> KNSINTIKLIDDIIALHNDPKGNKLLWNDNWQDKIINRDLANIFEKIDESVSELGGLEMYQEMVGVNPYDPTEPVCGLSAQNIFKLMTEGEHAVDPVEMAQTGKIDGNEFAESVDQLSSAKNYVALVNDRRLGHMFLIDIPSNDQETVGYIYQSDLGQGALPPLKIADWLNSRGKDAVSLNK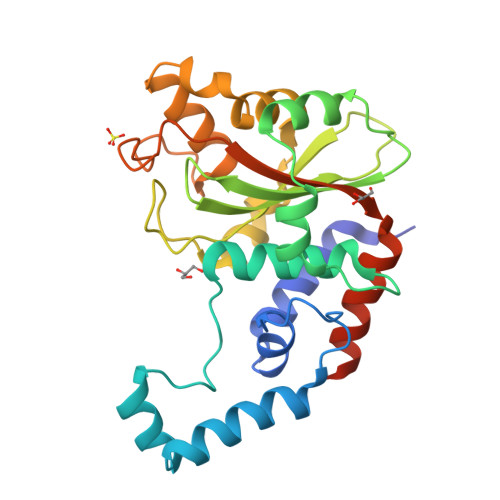LKKLLSREFNLLSDDEKRALISETLDIHKDVSNVELDRIKRDRGVDIYLTEYDVNNFYENIETLKSKLSNYDKKLSKPK> NTIELFYMPSDEELTANPNALQEASFTEEDINGLKGVDGVKQVVASAVKSMTARYHEEDTDITLNGINSGYMDVKKLDVQDGRTFTDNDFLSGKRAGIISKKMAEKLFGKTSPLGKIVWAGGQPVEVIGVLKEESGFLSLGLSEMYVPFNMLKTSFGTNDYSNVSVQTESADQIKSTGKEAARLLNDNHGTKEAYQVMN

The four-component transporter YknWXYZ in Bacillus has been implicated in the protection against SDP-dependent killing by expelling invading SDP toxin from the cytosol. YknWXYZ contains the ATP-binding cassette (ABC) transporter YknYZ, in which an individual protein YknY dimer associates with a respective permease (YknZ) that utilizes ATP hydrolysis as a driving force. The activity of YknYZ strictly depends on two accessory proteins, YknX and YknW. Unlike most dimeric ABC-type transporters, MacB and YknYZ are characterized as non-canonical ABC-type transporters, which consist of a four-transmembrane segment, an N-terminal nucleotide binding domain (NBD), and a large periplasmic domain.

Here, we present the first crystal structure of the extracellular domain of YknZ from Bacillus amyloliquefaciens. From the diffraction dataset, the crystals were found to belong to the orthorhombic space group P212121, with unit-cell parameters of a = 44.2, b = 46.2, and c = 87.5 Å. The refined model of Ba YknZ ED contains 188 residues from Asn58 to Asn256, and the N- and C-terminal regions of Ba YknZ ED were disordered in the crystal. The YknZ ED structure included a mixed α/β domain that was dispersed into upper and lower subdomains. The upper subdomain was formed by residues 103–219 and was composed of a seven-stranded antiparallel β-sheet with four α-helices. The lower subdomain was formed by residues 58–102 and 219–256 and consisted of three α-helices and a three-stranded antiparallel β-sheet. The DaliLite server revealed that the structure of Aa MacB PCD was highly similar to Ba YknZ ED, which was found to be the top match and showed a Z-score of 20.1 and sequence identity of up to 22%. We also found this crevice in the middle of the mixed α/β domain in the Ba YknZ ED structure, where it virtually divided the domain into two parts (Upper-right). The most significant structural difference is the number of β-strands; the lower subdomain of Ba YknZ ED contained three β-strands, while the other structures each contain four β-strands. The purified YknX protein was not bound to the CNbr-activated region, which is in sharp contrast to the strong binding of YknX to YknZ ED.> GSHMFLEDSELCWDTAAGSAKSCLSVRYDTVGNKTELDLKQIDVVSAKGLSFESDGKTKTPVVSTYETFQDGGRAKTINAIECPTGLNNRFAA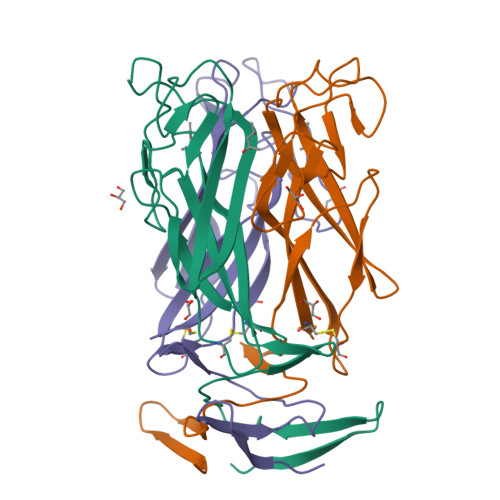VVSSFSTAGQNANFSSESAKDSQGTTQKDGSKGPHALLSGISLNWTLTNKVWDVTASIGIESGILPTSGIDSGSLLRNPKSLSFIAFQWCEN>CPRFLKVKNWETDVVLTDTLHLKSTLETGCTEHICMGSIMLPSQHTRKPEDVRTKDQLFPLAKEFLDQYYSSIKRFGSKAHMDRLEEVNKEIESTSTYQLKDTELIYGAKHAWRNASRCVGRIQWSKLQVFDARDCTTAHGMFNYICNHVKYATNKGNLRSAITIFPQRTDGKHDFRVWNSQLIRYAGYKQPDGSTLGDPANVQFTEICIQQGWKAPRGRFDVLPLLLQANGNDPELFQIPPELVLEVPIRHPKFDWFKDLGLKWYGLPAVSNMLL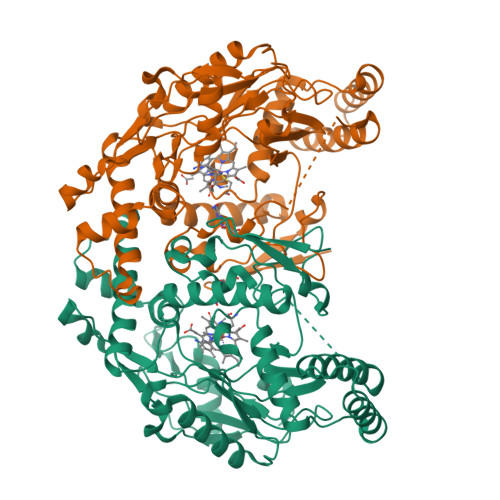EIGGLEFSACPFSGWYMGTEIGVRNYCDNSRYNILEEVAKKMDLDMRKTSSLWKDQALVEINIAVLYSFQSDKVTIVDHHSATESFIKHMENEYRCRGGCPADWVWIVPPMSGSITPVFHQEMLNYRLTPSFEYQPDPWNTHVWKG[2x]> RSQAPLSWEDITGKGLKQALDSCQQSFQWQRWNCPSQDFVQKNSKPEENSPNREDVYVAAISMAAIVHTLTKDCANGVIAGCGCTENALNVPCAHEPTKALEQYEKHFGSGSGAIGHNRRVVGALLQRSLEQECRCKQPGAVQGECQEEECVAVLKPFEAIAQDLLQMYDDAIQLEGASSNLKIMWQNIPLDSLVFMQDSPNYCERDATGLWGTG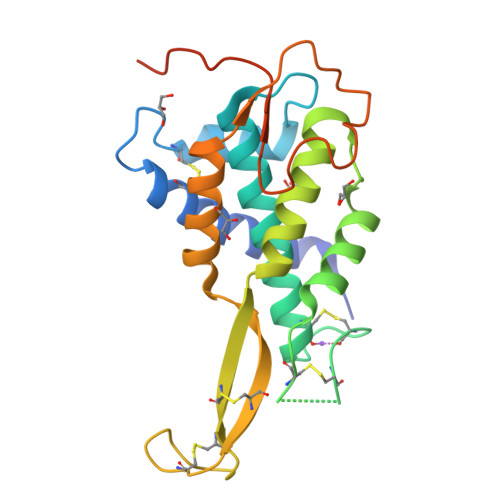HHHHHH>[3x]MTSTVSTDGPVYREYKGFRVNDNIVADFIGVPAVITPGETIEFSVFYTNRGRYAYPDTGLNLVIWFSDRDDLRREDFKLFYKVSRADWQEQDPAKCWDPQFPAEGGVHIACQLSGPDGGILSKPDGTVPLPEVESVTAHVRLAFREGITSEHAGIFALPGMLDAPGDKSIIPGLFGNVFGRLQQASFRLGEGPSSLY

In this work, we report the identification and characterization of a small enzyme AvmM that can catalyze the construction of a 16-membered macrocyclic ring in the biosynthesis of alchivemycin A. We show through in vivo gene deletion, in vitro biochemical assay and isotope labelling experiments that AvmM catalyzes tandem dehydration and Michael-type addition to generate the core scaffold of 1. Consistent with the apparent molecular weight (66.2 kDa) determined by the gel-filtration analysis, AvmM was characterized as a homotrimer, with each monomer adopting a jelly roll fold. The overall monomeric structure comprises of eight main β-strands arranged in two parallel four-stranded sheets, and three small β sheets. Using the DALI search program, AvmM shares low structural similarities to some components of large proteins, all of which adopted a jelly roll fold. Additionally, AvmM has a long C-terminal loop, which interacts with adjacent monomers to stabilize its quaternary structure.

Exhaustive efforts to get AvmM in complex with the substrate 3 by optimizing protein/ligand concentrations, pH values, temperatures, precipitant concentration or even rescreening the crystal condition were not successful, probably due to the relatively low binding affinity. However, we were able to obtain the complex structure of AvmM with the product 2 in a resolution of 2.5 Å. The overall structure of AvmM-2 complex is highly similar to the AvmM apo-form with a r.m.s.d. value of 0.18 Å for 574 Cα atoms. The enhanced polder omit map shows a clear electron density for product 2 in the active site. The rigid cis-decalin system interacts with F18, W97, I171, F179 and L182 through hydrophobic interaction, while H108 shows a weak hydrogen bonding with C3 carbonyl group. Additionally, residue Y15 was found to form a T-shaped π–π stacking interaction with the tetramic acid moiety. Furthermore, analyzing the B-factor of AvmM structures indicated that the loop1 and loop2 in chain A are highly flexible, and clear deviations of Y15, K16 in loop1 and E104, H108 in loop2 were observed by comparing chains A between the apo and complex structures. Importantly, the orientation of the docked substrate 3 is highly consistent with 2 in the active site of AvmM-2 complex structure. More importantly, the OH-23 hydroxyl is in a syn periplanar to the pro-R hydrogen at C-24, thus after syn-elimination, the specific twisted 3 would generate a Z-type C23 = C24 double bond. Interestingly, comparison of the docking result with crystal complex suggested that the formation of 16-member ring causes the polyketide side chain to move away from Chain B of the protein, disrupting the hydrogen bonds observed in the docking results. The formation of the 16-membered macrocyclic ring makes 2 more rigid and dramatically changes the conformation of flexible side chain in 3.> MGSSHHHHHHSSGRENLYFQGLPSINPHKKTIILSGAPNVGKSSFMNIVSRANVDVQS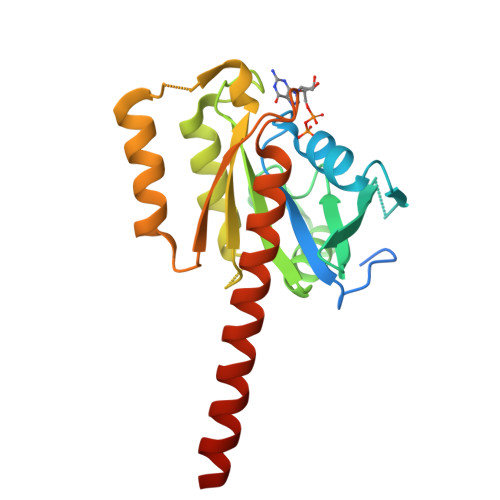YSFTTKNLYVGHFDHKLNKYQIIDTPGLLDRAFENRNTIEMTTITALAHINGVILFIIDISEQCGLTIKEQINLFYSIKSVFSNKSIVIGFNKIDKCNMDSLSIDNKLLIKQILDNVKNPIKFSSFSTLTGVGVEQAKITACELLKNDQAESILLDQEQLLNTKLGETKN>MAKKTSSKGKLPPGPTPLPFIGNYLQLNTEQMYNSLMKISERYGPVFTIHLGPRRVVVLCGHDAVKEALVDQAEEFSGRGEQATFDWLFKGYGVAFSNGERAKQLRRFSIATLRGFGVGKRGIEERIQEEAGFLIDALRGTHGANIDPTFFLSRTVSNVISSIVFGDRFDYEDKEFLSLLRMMLGSFQFTATSTGQLYEMFSSVMKHLPGPQQQAFKELQGLEDFIAKKVEHNQRTLDPNSPRDFIDSFLIRMQEEEKNPNTEFYLKNLVMTTLNLFFAGTETVSTTLRYGFLLLMKHPEVEAKVHEEIDRVIGKNRQPKFEDRAKMPYTEAVIHEIQRFGDMLPMGLAHRVNKDTKFRDFFLPKGTEVFPMLGSVLRDPRFFSNPRDFNPQHFLDKKGQFKKSDAFVPFSIGKRYCFGEGLARMELFLFFTTIMQNFRFKSPQSPKDIDVSPKHVGFA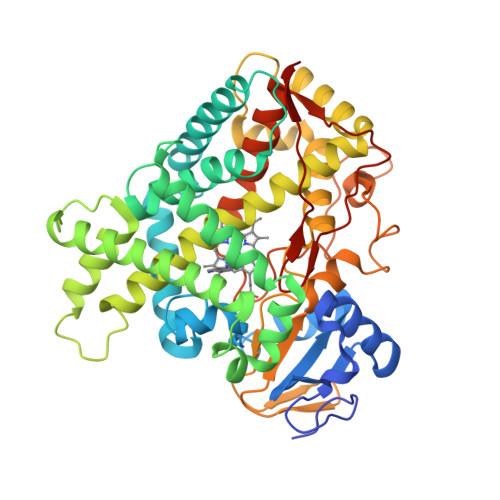TIPRNYTMSFLPRHHHH[6x]> MKPLSSPLQQYWQTVVERLPEPLAEESLSAQAKSVLTFSDFVQDSVIAHPEWLTELESQPPQADEWQHYAAWLQEALCNVSDEAGLMRELRLFRRRIMVRIAWAQTLALVTEESILQQLSYLAETLIVAARDWLYDACCREWGTPCNAQGEAQPLLILGMGKLGGGELNFSSDIDLIFAW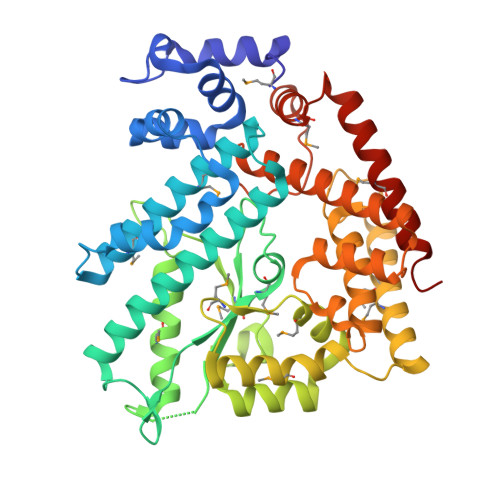PEHGCTQGGRRELDNAQFFTRMGQRLIKVLDQPTQDGFVYRVDMRLRPFGESGPLVLSFAALEDYYQEQGRDWERYAMVKARIMGDSEGVYANELRAMLRPFVFRRYIDFSVIQSLRNMKGMIAREVRRRGLTDNIKLGAGGIREIEFIVQVFQLIRGGREPSLQSRSLLPTLSAIAELHLLSENDAEQLRVAYLFLRRLENLLQSINDEQTQTLPSDELNRARLAWAMDFADWPQLTGALTAHMTNVRRVFNELIGDDE> MNVLALDTSQRIRIGLRKGEDLFEISYTGEKKHAEILPVVVKKLLDELDLKVKDLDVVGVGIGPGGLTGLRVGIATVVGLVSPYDIPVAPLNSFEMTAKSCPADGVVL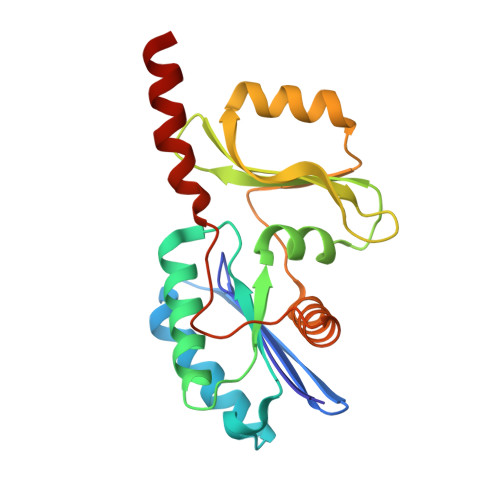VARRARKGYHYCAVYLKDKGLNPLKEPSVVSDEELEEITKEFSPKIVLKDDLLISPAVLVEESERLFREKKTIHYYEIEPLYLQKSIAELNWEKKKRG The sigma-1 receptor (σ1R) is a non-opioid transmembrane receptor which has been implicated in many diseases, including neurodegenerative disorders and cancer. The sigma-1 receptor (σ1R) is a small, unique integral membrane receptor that is localized primarily in the endoplasmic reticulum (ER). σ1R responds to a structurally diverse array of synthetic ligands such as (+)-pentazocine (agonist) and haloperidol (antagonist). Published structures of human σ1R reveal its homotrimeric organization of a cupin-fold β-barrel body that contains the ligand binding site, a carboxy-terminal V-shaped two-helix bundle, and a single amino-terminal transmembrane helix, while simulation studies have suggested a ligand entry pathway that is generated by conformational rearrangements of the cupin-fold domain. Here, we present multiple crystal structures, including an open-like conformation, of σ1R from Xenopus laevis. Together with functional binding analysis our data suggest that access to the σ1R ligand binding site is likely achieved by protein conformational changes that involve the carboxy-terminal two-helix bundle, rather than structural changes in the cupin-fold domain.

In the end, we solved a structure for the wild-type σ1R from Xenopus laevis (xlσ1R), which shares 67% sequence identity and 89% sequence homology with human σ1R (hσ1R), to 3.20 Å, and termed it xlσ1Rclosed-endo. The xlσ1Rclosed-endo structure was solved in the space group P21 with each asymmetric unit containing 12 protomers, which deviate little from each other with all-atom RMSDs of only ~0.2 Å between the protomers. Superposition of individual protomers of xlσ1Rclosed-endo and hσ1RPD144418 excluding α1 yielded an all-Cα RMSD of 0.35 Å, indicating a high degree of structural conservation among σ1Rs from different species. However, xlσ1Rclosed-endo failed to achieve our initial goal as it was captured in a closed conformation similarly to hσ1RPD144418. Surprisingly, though no known ligand was added during purification or crystallization of xlσ1R, a clear electron density within the ligand-binding pocket indicates that xlσ1Rclosed-endo was bound by an unknown molecule, which may have an endogenous origin. Unfortunately, the current resolution of xlσ1Rclosed-endo (3.20 Å) provides only limited details about the shape of the electron density, making it impossible to reveal readily the molecular identity of this unknown molecule, and therefore the electron density was not modeled in xlσ1Rclosed-endo. In each asymmetric unit of xlσ1Rclosed-endo there are four homotrimers of xlσ1R, which are organized in a diamond shape with the cupin-fold domains packing against each other, whereas the transmembrane helices (α1s) mediate crystal contacts between adjacent asymmetric units. In such a packing mode, each trimer has one protomer whose cupin-fold domain is tightly buried by two adjacent cupin-fold domains.

>[12x]SVDTMALWLGLRAVLVVAGLAVLLQLIRGWLSSKSYVFNREEIARLAKEHSGLDYEVAFSKIIVELRKKHPGHILQDEDLQWVFVNAGGWMGSMCLLHASLTEYVLLFGTAVDTGGHSGRYWAEISDTILSGTFRQWKEGTTKSEIFYPGDTIVHEVGEATSVQWSSGTWMVEYGRGFIPSTLAFALADTIFSTQDFLTLFYTVKVYSKALLLEASTHLSQLGFF Carbamate kinase (CK; EC 2.7.2.2, ATP:carbamate phosphotransferase) reversibly converts ADP and carbamoyl phosphate into ATP and ammonium carbamate. The enzyme functions in the L-arginine dihydrolase pathway, operative primarily in some bacteria but also in the enteric protozoan parasite, Giardia lamblia. CK assembles into homodimers, consistent with the oligomeric form detected in solution. Each subunit contains an eight-stranded β-sheet surrounded by three α-helices on one side and four α-helices on the other side of the β-sheet.

A citrate ion occupies each subunit of the glCK homodimer in both glCK-citrateS and glCK-citrateL complexes. The main difference between the two structures is in the conformational state of one of the auxiliary domains. In the glCK-citrateS structure, all four auxiliary domains in the asymmetric unit are placed in proximity to the bound citrate, a state referred to as the closed conformation. In both glCK-citrate and efCK-SO4 structures the auxiliary domains are in the closed conformations, and the closure partially protects the ligands from bulk solvent. As with the nitrogen atom of the AMP-PNP β,γ-imidophosphate, the C5-carboxylate of citric acid interacts with the backbone nitrogen of Gly13. The C6 carboxyl group also interacts with Lys131’s amino group, located on the auxiliary domain. Finally, the C1 carboxyl group is bridged to Arg163 on the auxiliary domain via a water molecule.

>[4x]GMSAGKTVVIALGGNAMLQAKEKGDYDTQRKNVEIAASEIYKIHKAGYKVVLTSGNGPQVGAIKLQNQAAAGVSPEMPLHVCGAMSQGFIGYMMSQAMDNVFCANNEPANCVTCVTQTLVDPKDQAFTNPTKPVGRFYTEQEAKDLMAANPGKILREDAGRGWRVVVPSPRPLEIVEYGVIKTLIDNNVLVICTNGGGIPCKRENKVISGVDAVIDKDLATSLLAKTLNSDYLMILTDVLNACINYKKPDERKLEEIKLSEILALEKDGHFAAGSMGPKVRAAIEFTQATGKMSIITSLSTAVDALNGKCGTRIIKD>[2x]GKATTEEQKLIEDVNASFRAAMATTANVPPADKYKTFEAAFTVSYKRNLADAVSKA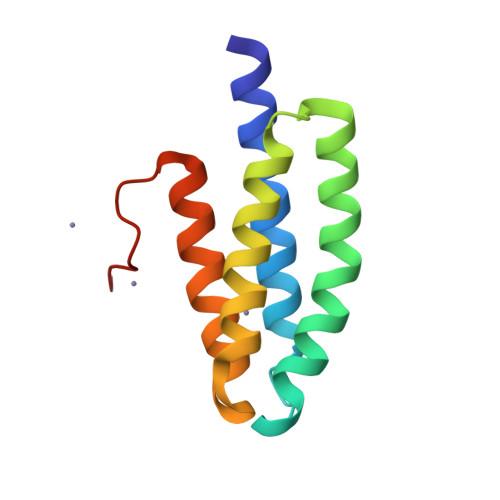PQLVPKLDEVYNAAYNAADHAAPEDKYEAFVLHFSEALRIIAGTPEVHAVKPGA I-CreI is a homodimeric member of LHEs family, which recognizes and cleaves a 22 bp pseudo-palindromic target (5′- CAAAACGTCGTGAGACAGTTTG -3′). Each I-CreI monomer binds its own DNA target region generating the catalytic centre at the dimer interface. This region contains two catalytic aspartic acids (D20, one per each monomer). The aspartic side chains participate in the cleavage of the DNA strands along the minor groove, resulting in the hydrolysis of specific phosphodiester bonds upon the coordination of three divalent metal ions.

Thus, a 24 bp palindromic DNA target is recognized and cleaved by a I-CreI variant (I-CreI D75N) with similar affinity and activity than in the wild-type case. The absence of the central metal ion in the non-cleaved structures, would explain the different catalytic behaviour. To assess unambiguously the number of catalytic ions present in the active site, we solved the crystal structure of the two proteins in complex with both target DNAs in the presence of Mn2+, which allows catalysis and unambiguous detection and location through its anomalous diffraction signal. In-depth analysis showed differences in the occupancy of the central metal at the active site between cleavable and non-cleavable targets. A high occupancy level of the central metal ion is essential for the cleavage, and the lower occupancy level of the central Mn2+ ion found in the non-cleavable targets (46% and 74% for I-CreI_D75N_target-null and I-CreI_3115_target-null, respectively) compared with the cleavable ones (100% in both cases) revealed that the non-cleavable targets interfere with the positioning of the central metal ion affecting catalysis. On the other hand, when the two enzyme variants were simulated bound to the I-CreI_D75N_target and I-CreI_3115_target DNA sequences, the helical parameters of A +1 were similar to those found in the ideal B-DNA conformation, with minor fluctuations typical of atomic thermal motions.

>NTKYNKEFLLYLAGFVDGDGSIIAQIKPNQSYKFKHQLSLTFQVTQKTQRRWFLDKLVDEIGVGYVRDRGSVSNYILSEIKPLHNFLTQLQPFLKLKQKQANLVLKIIEQLPSAKESPDKFLEVCTWVDQIAALNDSKTRKTTSETVRAVLD[2x]>MKFAEHLSAHITPEWRKQYIQYEAFKDMLYSAQDQAPSVEVTDEDTVKRYFAKFEEKFFQTCEKELAKINTFYSEKLAEAQRRFATLQNELQSSLDAQKESTGVTTLRQRRKPVFHLSHEERVQHRNIKDLKLAFSEFYLSLILLQNYQNLNFTGFRKILKKHDKILETSRGADWRVAHVEVAPFYTCKKINQLISETEAVVTNELEDGDRQKAMKRLRVPPLGAAQ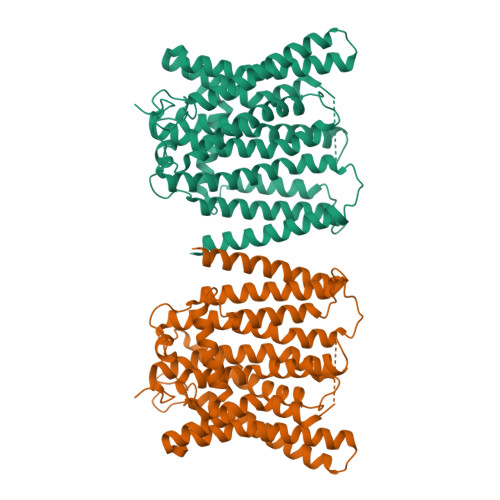PAPAWTTFRVGLFCGIFIVLNITLVLAAVFKLETDRSIWPLIRIYRGGFLLIEFLFLLGINTYGWRQAGVNHVLIFELNPRSNLSHQHLFEIAGFLGILWCLSLLACFFAPISVIPTYVYPLALYGFMVFFLINPTKTFYYKSRFWLLKLLFRVFTAPFHKVGFADFWLADQLNSLSVILMDLEYMICFYSLELKWDESKGLLPNNSEESGICHKYTYGVRAIVQCIPAWLRFIQCLRRYRDTKRAFPHLVNAGKYSTTFFMVTFAALYSTHKERGHSDTMVFFYLWIVFYIISSCYTLIWDLKMDWGLFDKNAGENTFLREEIVYPQKAYYYCAIIEDVILRFAWTIQISITSTTLLPHSGDIIATVFAPLEVFRRFVWNFFRLENEHLNNCGEFRAVRDISVAPLNADDQTLLEQMMDQDDGVRNRQKNRSWKYNQSISLRRPRLASQSKARDTKVLIEDTDDEANTENLYFQGHHHHHHHHSGAAAWSHPQFEK[2x]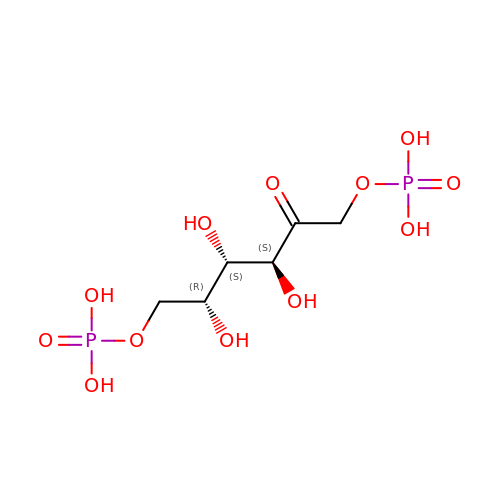1,6-di-O-phosphono-D-tagatose | C6 H14 O12 P2 | XPYBSIWDXQFNMH-PQLUHFTBSA-N>MVSEYIDSELKRLEDYALRRVKGIPNNRRLWVLTCMDERVHIEQSLGIQPDDAHIYRNAGGIVTDDAIRSASLTTNFFGTKEIIVVTHTDCGMLRFTGEEVAKYFISKGIKPTEVQLDPLLPAFRISSEEDFIKWFKF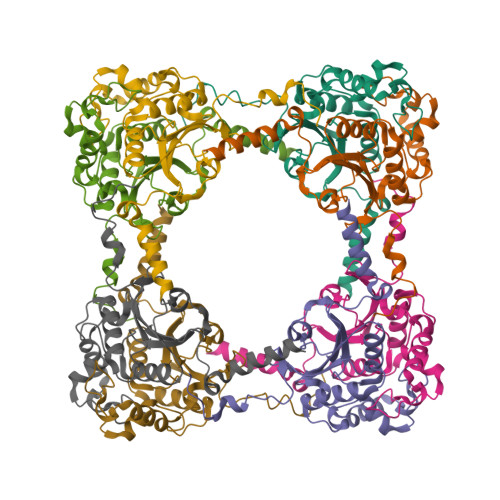YEDLGVKSPDEMALKGVEILRNHPLIPKDVRITGYVYEVETHRLRKPNQIIYNETSKFEHGTIVKE[8x]>[4x]MSTLYSTQVKAVGGCSGTIRSEDGILELKLALPKELGGKGDATNPEQLFAAGYAACFGN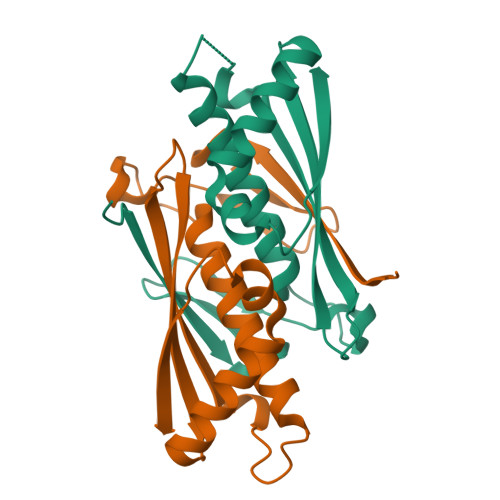AVIHVTRSNKEYKIRDNDVEVLSTVGIVANGNGGFALTVHLDVTLSGISQADAEKIVEQTHQVCPYSNAIRGNIQVSTTVYTK> MATLRIGLVSISDRASSGVYQDKGIPALEEWLTSALTTPFEL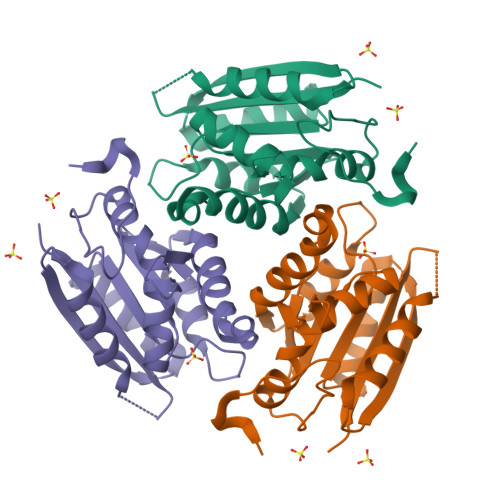ETRLIPDEQAIIEQTLCELVDEMSCHLVLTTGGTGPARRDVTPDATLAVADREMPGFGEQMRQISLHFVPTAILSRQVGVIRKQALILNLPGQPKSIKETLEGVKDAEGNVVVHGIFASVPYCIQLLEGPYVETAPEVVAAFRPKSARRDVSE>MELRHLRYFVAVVEEQSFTKAADKLCIAQPPLSRQIQNLEEELGIQLLERGSRPVKTTPEGHFFYQYAIKLLSNVDQMVSM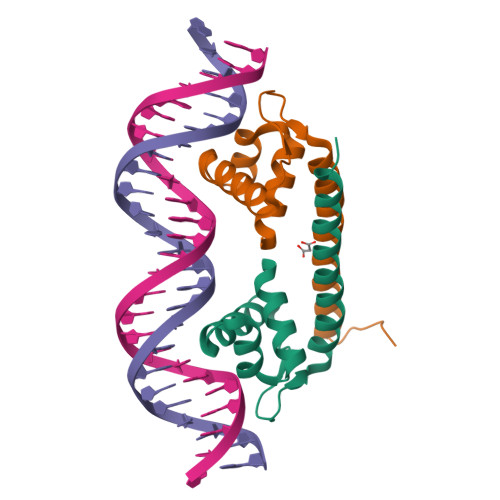TKRIASGHHHHHH[4x]1-[4-ethyl-2-methyl-5-(2-piperazin-1-yl-1,3-thiazol-4-yl)-1~{H}-pyrrol-3-yl]ethanone | C16 H22 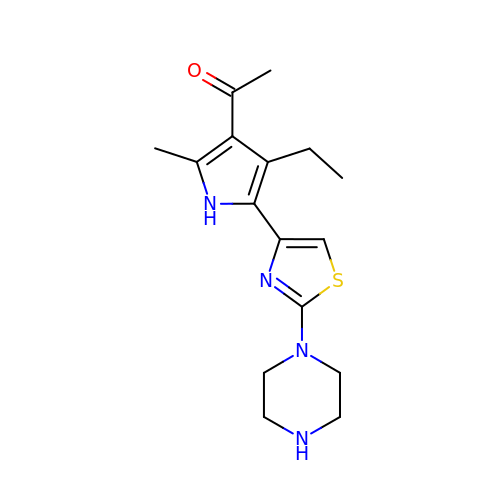N4 O S | GSMRYQUEJCTMHR-UHFFFAOYSA-N> MTKSKMLSNIVIQEVKFAIED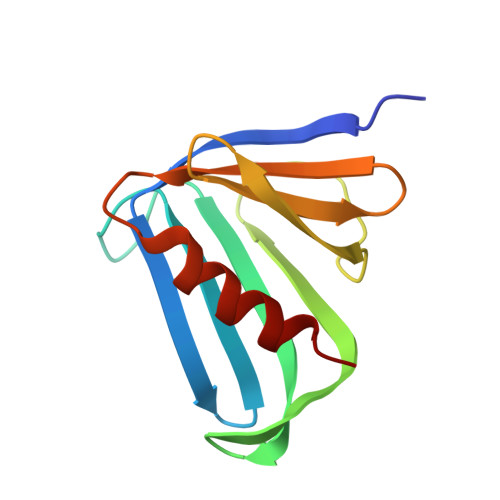YCAILSFASDSYEVPEQYFIITRSTTERSGGIPEGDIYLESNLFLDFNPYGLSGYLLSEPNCVDLLIEPNNYVRLRLIEKIDILEVENHLKFLFDN The ESCRT machinery mediates membrane remodeling in numerous processes in cells including cell division and nuclear membrane reformation. The identification of ESCRT homologs in Asgard archaea, currently considered the closest prokaryotic relative of eukaryotes, implies a role for ESCRTs in the membrane remodeling processes that occurred during eukaryogenesis. Here we show that Asgard ESCRT-III proteins of the Lokiarcheota self-assemble into helical filaments, a hallmark of the ESCRT system. Notably, the Asgard ESCRT-III subfamily is substantially reduced compared to eukaryotes with only two ESCRT-III proteins (named here CHMP1-3 and CHMP4-7) encoded in some species including Loki and Heimdall archaeota.

Next, we determined the cryo-EM structure of helical CHMP4-7 tubes in the presence of CHMP1–3 and DNA at a resolution of 3.6 Å. We were able to determine the structure of 36 nm PspA-like rods at a global resolution of 3.6 Å and a local resolution ranging from 3.0 Å at the inner rod wall to 6.0 Å at the outer tube wall. The rods are arranged by helical symmetry with 1.05 Å rise and 173.9° rotation. Thus we, relied on the strong density to build a model for Loki CHMP4-7 α1–5 into the density, while no density was found for helices α0 and α6. CHMP1-3 is, therefore, not a regular member of the symmetric rod assemblies while it may be part of the curved filaments, involved in nucleation or occasionally bound to the rod assemblies. The structured elements of CHMP4-7 adopt the canonical ESCRT-III fold: α1–3 form an extended hairpin, connected to α4 via a short linker (E117-P120 Fig. 5B, inset). Helix α4 is separated in two parts by a short loop at G146 and connected to α5 by an extended linker (I154-E159). The monomers are arranged in a j + 4 repeat, where α5 of chain j packs perpendicularly against the tip of the hairpin of j + 4, forming the typical ESCRT-III assembly motif known from IST1/CHMP1B. In the assembly, helices α1-4 make up the wall of the rods, while α5 together with the tip of the α1 + 2 hairpin forms the spikes on the outside of the wall. In CHMP4-7 rods of Asgard, α5 only interacts with a single hairpin at the bottom end, which is a common feature in eukaryotic ESCRT-III assemblies, while in bacteria top and bottom ends of α5 are interacting with two hairpins connecting two layers of the assembly (bottom). Therefore, the Loki CHMP4-7 assembly more closely resembles the bacterial configuration with the characteristic spike, while the Loki CHMP4-7 monomer adopts a conformation closer to previously determined eukaryotic structures including the α1/2-α5 interaction motif.

> MGLKKKLFPRKKGKEKANLITNAKVHIHKLNLVNRNYTKRAEISRKNAKIALRRGEKTRAKNFLIQYKSYNAKIDRSNNIRSKIERQIQAIEEGQLISQTGSIFEGIRDELKYIATEASPAKVAEIAEDSDVYVSEIEEAADILAGDPEIDLGIDVTDELNQLETELLLSQGGTMPDAPSDDLQYIPEYGDELEEEVESKTKEKVQAEIEKLRKELES>MGVDPFERNKILGRGINIGNALEAPNEGDWGVVIKDEFFDIIKEAGFSHVRIPIRWSTHAYAFPPYKIMDRFFKRVDEVINGALKRGLAVVINIHHYEELMNDPEEHKERFLALWKQIADRYKDYPETLFFEILNEPHGNLTPEKWNELLEEALKVIRSIDKKHTIIIGTAEWGGISALEKLSVPKWEKNSIVTIH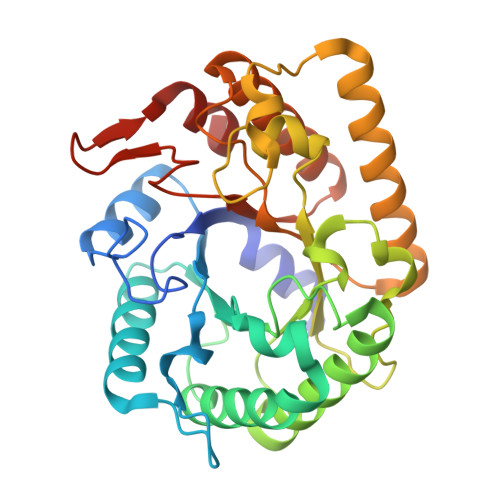YYNPFEFTHQGAEWVEGSEKWLGRKWGSPDDQKHLIEEFNFIEEWSKKNKRPIYIGEFGAYRKADLESRIKWTSFVVREMEKRRWSWAYWEFCSGFGVYDTLRKTWNKDLLEALIGGDSIE[4x]> MSTGDFLTKGIELVQKAIDLDTATQYEEAYTAYYNGLDYLMLALKYEKNPKSKDLIRAKFTEYLNRAEQLKKHLESEEANAAKKSPSAGSGSNGGNKKISQEEGEDNGGEDNKKLRGALSSAILSEKPNVKWEDVAGLEGAKEALKEAVILPVKFPHLFKGNRKPTSGILLYGPPGTGKSYLAKAVATEANSTFFSVSSSDLVSKWMGESEKLVKQLFAMARENKPSIIFIDQVDALTGTRGEGESEASRRIKTELLVQMNGVGNDSQGVLVLGATNIPWQLDSAIRRRFERRIYIPLPDLAARTTMFEINVGDTPCVLTKEDYRTLGAMTEGYSGSDIAVV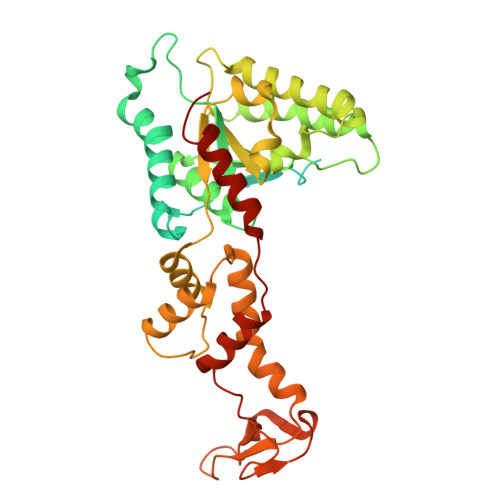VKDALMQPIRKIQSATHFKDVSTEDDETRKLTPCSPGDDGAIEMSWTDIEADELKEPDLTIKDFLKAIKSTRPTVNEDDLLKQEQFTRDFGQEGN>[2x]MGEDDKLKRMFSWSSNALSEGSAMGERVEPVVPGPDLVGVNVERPPAPLVHQQSTVWSKRQHAVCVRHAFKQYGSKKNPNHVLSDLNMTVAKGTIYGLLGASGCGKTTLLSCIVGRRRLNTGEIWVLGGKPGTKGSGVPGKRVGYMPQEIALYGEFSI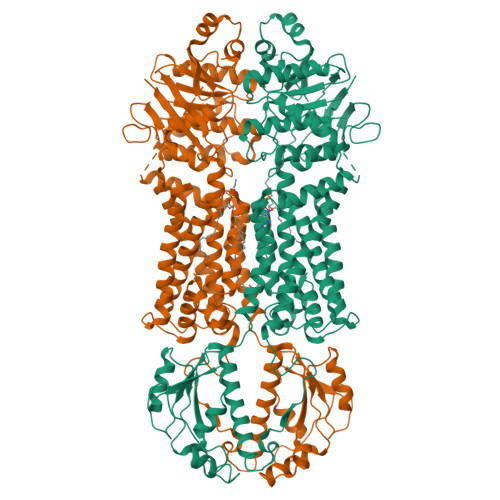KETMMYFGWIFGMESSEINERLQFLLNFLDLPSQNRLVKNLSGGQQRRVSFAVALMHDPELLILDEPTVGVDPLLRQSIWNHLVQITKDGNKTVIITTHYIEEARQAHTIGLMRSGKLLAEESPHVLLSMYGCQSLEEVFLKLSRKQGQANQNDINISNNISLATLNWGKKDSISVTEESGVVGLNFHQSKEILIADSTNGHIDLNGLGKPSSSKSSMADACDDCSCSDMTSWGKIKALLQKNFLRMWRNVGVMLFIFALPVMQVILFCLAIGRDPTGLKLAIVNHEKNYTNQSYQECSFDYGCKFSYLSCRYLNNLRNSTILKEYYPDPESAVDAVKQGHAWGALYFTENFTDALVARMALGKDADPETLDQSEVRVWLDMSNQQIGIILQRDLQLSYQDFAKDLLGACEQNPDLAEIPISFKEPIYGSNKPSFTDFVAPGVILTIVFFLAVALTSSALIIERMEGLLDRSWVAGVTPGEILFSHVVTQFVVMCGQTALVLIFMILVFGVQCKGDIGWVIVLTILQGLCGMCFGFVISAICELERNAIQLALGSFYPTLLLSGVIWPIEGMPTVLRYVSTFLPLTLATTSLRAMLTRGWSIAEPAVYYGFLATIIWIVAFLTISMLVLRFKRG> MGMTGHHGWGYGQDDGPSHWHKLYPIAQGDRQSPINIISSQAVYSPSLQPLELSYEACMSLSITNNGHSVQVDFNDSDDRTVVTGGPLEGPYRLKQFHFHWGKKHDVGSEHTVDGKSFPSELHLVHWNAKKYSTFGEAASAPDGLAVVGVFLETGDEHPSMNRLTDALYMVRFKGTKAQFSCFNPKSLLPASRHYWTYPGSLTTPPLSESVTWIVLREPISISERQMGKFRSLLFTSEDDERIHMVNNFRPPQPLKGRVVKASFRALEHHHHHH

Human carbonic anhydrase (CA; EC 4.2.1.1) isoforms II and VII are implicated in neuronal excitation, seizures, and neuropathic pain (NP). As CAs are implicated in maintaining the bicarbonate gradient that results in the efflux of HCO3– ions through GABAA receptors, this study corroborated the involvement of CA VII as well as CA II in neuronal excitation and seizures. In this study, by observing the significant similarity in amino acid composition and active site architecture existing between hCA II and hCA VII, a new series of CAIs were designed, which can concomitantly target both isozymes with the aim of achieving a neuropathic pain-relieving action. In detail, CA II and CA VII share a Phe residue in position 131.

CA VII is deemed a brain-associated CA isozyme as it is predominantly expressed in the CNS while missing in most other systems. To understand the molecular basis responsible for the inhibition efficiency of phosphonate/phosphonamidate benzenesulfonamides against CA II and CA VII, the crystal structure of these two isoforms was solved in adduct with phenylphosphonic acid 3. This compound based on the ChemAxon software36 has a pKa value of 1.62 and, therefore, is assumed to bind the enzyme at physiological pH and in crystallization conditions in a deprotonated, nonchiral form. Crystals of the CA adducts with 3 were obtained by soaking experiments as previously reported for other sulfonamide CA inhibitors. Data were collected to resolution values of 1.26 and 1.94 Å for CA II/3 and CA VII/3 complexes, respectively. The electron density maps were very well defined for both proteins and for the entire inhibitor in the case of CA VII/3. In detail, in both structures, the benzenesulfonamide moiety binds the active site in the same conformation adopted in other CA/benzenesulfonamide complexes, coordinating the catalytic zinc ion, forming two hydrogen bonds with residue Thr199, and establishing many hydrophobic interactions with residues located on the bottom of the cavity. The phosphonate group points toward the hydrophilic region of the active site13 and forms in both structures several water-mediated hydrogen bonds with enzyme residues. Finally, the phenyl tail is oriented toward the hydrophobic side of the active site13 establishing many hydrophobic interactions with residues delimiting this region and interacting with residue Phe131 as hypothesized in the design. The comparable number and nature of the interactions established by the inhibitor in the two active sites might explain the similarity of the inhibition constants against the two isoforms.> MIKSTGALLLFAALSAGQAIASDVAFRGNLLDRPCHVSGDSLNKHVVFKTRASRDFWYPPGRSPTESFVIRLENCHAT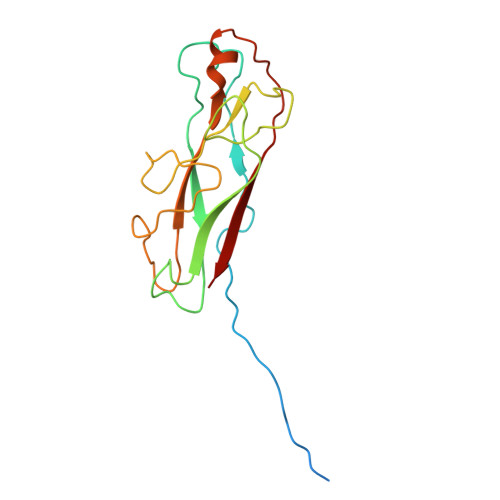AVGKIVTLTFKGTEEAALPGHLKVTGVNAGRLGIALLDTDGSSLLKPGTSHNKGQGEKVTGNSLELPFGAYVVATPEALRTKSVVPGDYEATATFELTYR> MKIKTIKRSADDYVP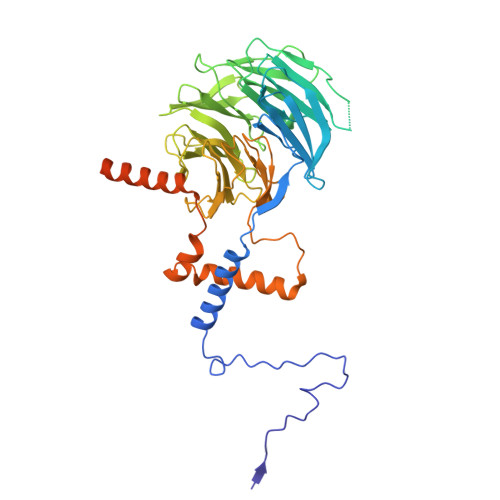VKSTQESQMPRNLNPELHPFERAREYTKALNATKLERMFAKPFVGQLGYGHRDGVYAIAKNYGSLNKLATGSADGVIKYWNMSTREEFVSFKAHYGLVTGLCVTQPRFHDKKPDLKSQNFMLSCSDDKTVKLWSINVDDYSNKNSSDNDSVTNEEGLIRTFDGESAFQGIDSHRENSTFATGGAKIHLWDVNRLKPVSDLSWGADNITSLKFNQNETDILASTGSDNSIVLYDLRTNSPTQKIVQTMRTNAICWNPMEAFNFVTANEDHNAYYYDMRNLSRSLNVFKDHVSAVMDVDFSPTGDEIVTGSYDKSIRIYKTNHGHSREIYHTKRMQHVFQVKYSMDSKYIISGSDDGNVRLWRSKAWERSNVKTTREKNKLEYDEKLKERFRHMPEIKRISRHRHVPQVIKKAQEIKNIELSSIKRREANERRTRKDMPYISERKKQIVGTVHKYEDSGRDRKRRKEDDKRDTQEK Calcium-activated chloride channels (CACC) facilitate transmembrane anion conduction in response to the increase of the intracellular Ca2+ concentration. The most prominent CACC is formed by TMEM16A, which is expressed in different tissues of the human body. Structures of both functional branches have revealed the general architecture of the family. These proteins form homodimers with subunits containing ten membrane-spanning segments. Our study reveals the location of a hydrophobic gate at the intracellular entry to the neck that controls ion conduction in TMEM16A thereby contributing to the tight regulation of its open probability.

Finally, we determined the structure of the mutant I551A in the absence of Ca2+ to elucidate the structural features underlying its activating behavior. The structure at 3.3 Å provides a detailed view of a constitutively active mutant in a ligand-free state. Whereas the mutant resembles WT in the Ca2+-bound state, the Ca2+-free structure of I551A exhibits pronounced differences compared to the corresponding structure of WT. Compared to the Ca2+-free wild-type structure where the intracellular part of α6 has moved towards α4, in I551A it moved outwards by about 30° in a direction away from α4, resembling a conformation that was also found for the Ca2+-free state of the lipid scramblase TMEM16F14. As for WT, the π-helical region of α6 located below the gating hinge Gly 644 found in the Ca2+-bound state has also relaxed towards a canonical α-helix in I551A, despite the difference in the conformation of α6 between the apo structures. The loss of density beyond Asn 651 in I551A presumably reflects the increased flexibility of the helix in the absence of Ca2+. The observed differences between the Ca2+-free structures of WT and I551A emphasize the functional interaction between the gate region and the intracellular half of α6 in TMEM16A. The relative stabilization of the open state in the mutant enables α6 to adopt a seemingly more activated conformation (with partially straightened helix α6), in part overcoming the electrostatic repulsion at the vacant Ca2+ binding site. Thus, it is conceivable that the observed structure displays features relevant to the mutant’s basal activity where, even in the absence of Ca2+, the movement of α6 couples to the narrow neck to stabilize a conductive state of the channel. Importantly, these observations suggest that pore opening can proceed without the transition of α6 into a straightened π-helix conformation.

>MRVPEKYSTLPAEDRSVHIVNICAIEDLGYLPSEGTLLNSLSVDPDAECKYGLYFRDGKRKVDYILVYHHKRASGSRTLARRGLQNDMVLGTRSVRQDQPLPGKGSPVDAGSPEVPMDYHEDDKRFRREEYEGNLLEAGLELENDEDTKIHGVGFVKIHAPWHVLCREAEFLKLKMPTKKVYHISETRGLLKTINSVLQKITDPIQPKVAEHRPQTTKRLSYPFSREKQHLFDLTDRDSFFDSKTRSTIVYEILKRTTCTKAKYSMGITSLLANGVYSAAYPLHDGDYEGDNVEFNDRKLLYEEWASYGVFYKYQPIDLVRKYFGEKVGLYFAWLGAYTQMLIPASIVGVIVFLYGCATVDENIPSMEMCDQRYNITMCPLCDKTCSYWKMSSACATARASHLFDNPATVFFSVFMALWAATFMEHWKRKQMRLNYRWDLTGFEEEEEAVKDHPRAEYEARVLEKSLRKESRNKETDKVKLTWRDRFPAYFTNLVSIIFMIAVTFAIVLGVIIYRISTAAALAMNSSPSVRSNIRVTVTATAVIINLVVIALLDEVYGCIARWLTKIEVPKTEKSFEERLTFKAFLLKFVNSYTPIFYVAFFKGRFVGRPGDYVYIFRSFRMEECAPGGCLMELCIQLSIIMLGKQLIQNNLFEIGIPKMKKFIRYLKLRRQSPSDREEYVKRKQRYEVDFNLEPFAGLTPEYMEMIIQFGFVTLFVASFPLAPLFALLNNIIEIRLDAKKFVTELRRPVAIRAKDIGIWYNILRGVGKLAVIINAFVISFTSDFIPRLVYLYMYSQNGTMHGFVNHTLSSFNVSDFQNGTAPNDPLDLGYEVQICRYKDYREPPWSEHKYDISKDFWAVLAARLAFVIVFQNLVMFMSDFVDWVIPDIPKDISQQIHKEKVLMVELFMREEQGKQQLLDTWMEKEKPRDVPCNNHSPTTHPEAGDGSPVPSYEYHGDAL[2x]> MATFTDAEIDELFE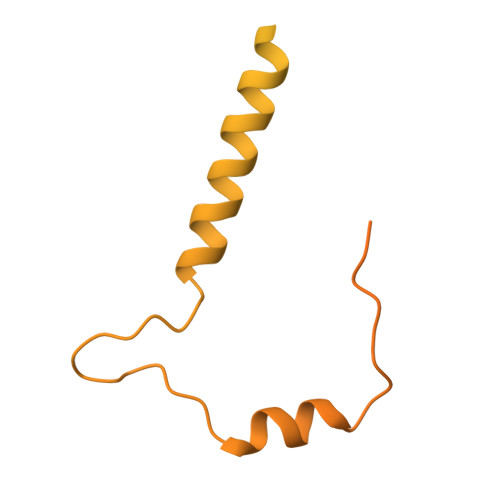TSGTVIDSIITAQGKPVETVGRSAIPQGKTKALSLAWEKHGNTNTPAAQESAGEQDQHGQNQASNSNRATPEEGPHSSQAQAATQPQEDANESQLKTGASSSLLSMLDKLSNKSSNAKKGPPQSPPQQALHSKGSPAVEQTQHGANQGRAQQETGHQAAPSPGPPGTGVNIAFPGQRGVSPQSVGATQPAPQSGQNQGSTPASADHVQPPVDFVQAMMSMMEAISQRVSKIDYQLDLVLKQTSSIPTMRSEIQQLKTSVAVMEANLGMMKILDPGCANVSSLSDLRAVAKSHPVLIAGPGDPSPYVTQGGEIALNKLSQPVPHPSDLIKHATSGGPDIGIERDTVRALILSRPMHPSSSSKLLSKLDSAGSVEEIRKIKRLALNG6-BROMOHEXAN-1-OL 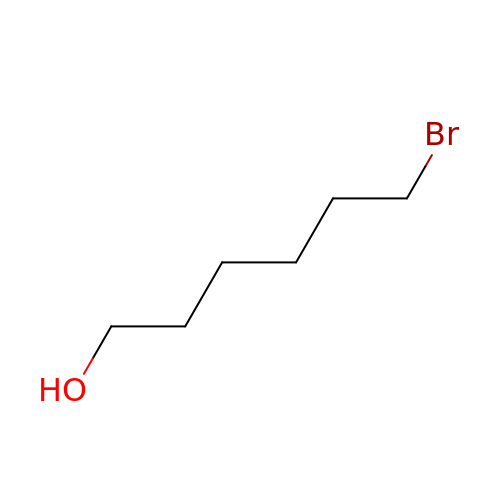| C6 H13 Br O | FCMCSZXRVWDVAW-UHFFFAOYSA-N>MRLEECNILFELLTEIQDEAGSMEKIVHKTLQRLSQLLAADRCSMFICRSRNGIPEVATRLLNVTPTSKFEDNLVNPDKETVFPLDIGIAGWVAHTKKFFNIPDVKKNNHFSDYLDKKTGYTTVNMMAIPITQGKEVLAVVMALNKLNASEFSKEDEEV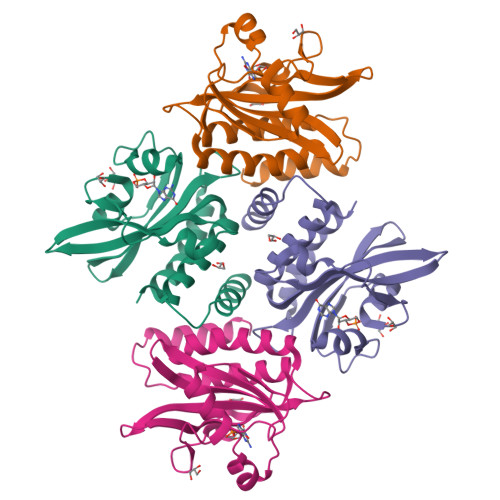FKKYLNFISLVLRLEHHHHHH[2x]> XGLCALRSELQALRREGFSPEELAALESELQALERELAALRSELQA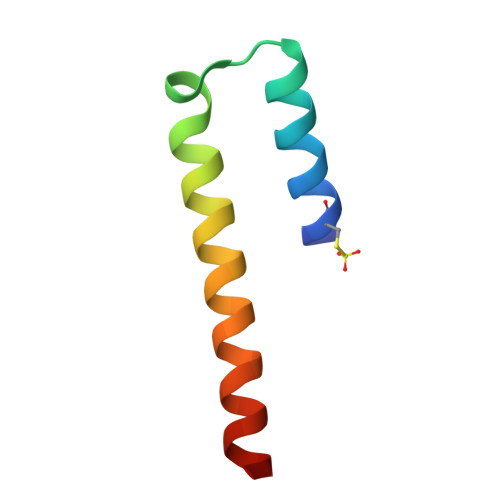LRGX>MKLLVLGTGGTIASAKTEMGYKAALSADDILQLAGIRREDGAKIETRDILNLDSTLIQPEDWVTIGRAVFEAFDEYDGIVITHGTDTLAYTSSALSFMIRNPPIPVVLTGSMLPITEPNSDAPRNLRTALTFARKGFPGIYVAFMDKIMLGTRVSKVHSLGLNAFQSINYPDIAYVKG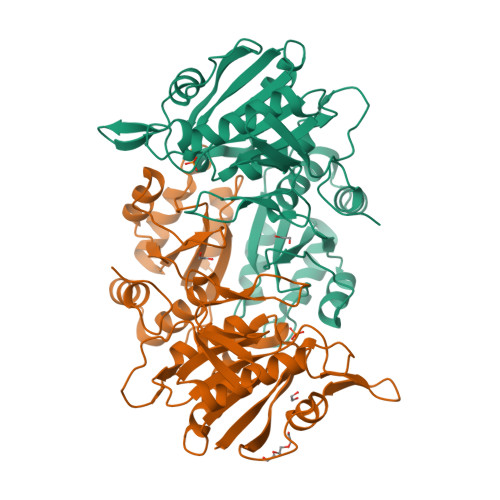DEVLVRHKPRIGNGEPLFDPELDPNVVHIRLTPGLSPEVLRAVARATDGIVLEGYGAGGIPYRGRNLLEVVSETAREKPVVMTTQALYGGVDLTRYEVGRRALEAGVIPAGDMTKEATLTKLMWALGHTRDLEEIRKIMERNIAGEITGS[6x]> MIPGGLSEAKPATPEIQEIVDKVKPQLEEKTNETYGKLEAVQYKTQVVAGTNYYIKVRAGDNKYMHLKVFKSLP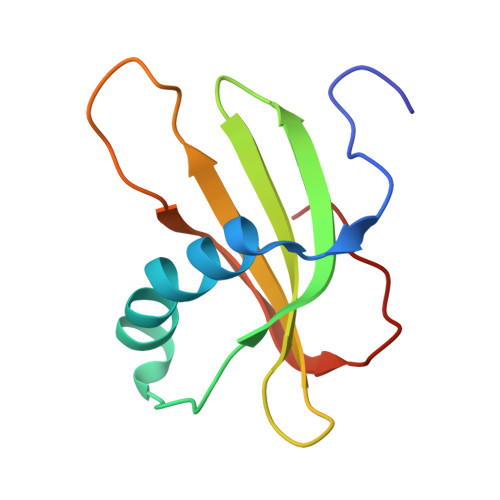GQNEDLVLTGYQVDKNKDDELTGF> MATSRYEPVAEIGVGAYGTVYKARDPHSGHFVALKS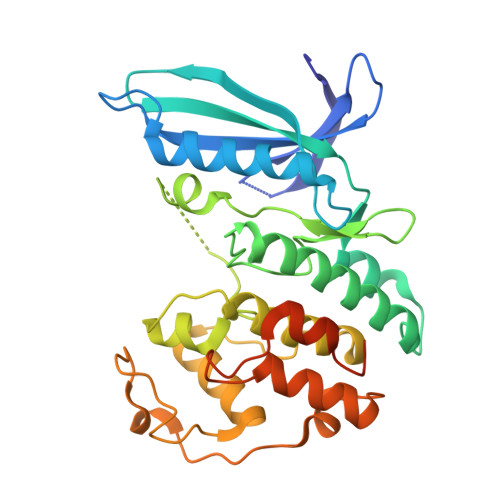VRVPNGEEGLPISTVREVALLRRLEAFEHPNVVRLMDVCATSRTDREIKVTLVFEHVDQDLRTYLDKAPPPGLPAETIKDLMRQFLRGLDFLHANCIVHRDLKPENILVTSGGTVKLADFGLARIYSYQMALTPVVVTLWYRAPEVLLQSTYATPVDMWSVGCIFAEMFRRKPLFCGNSEADQLGKIFDLIGLPPEDDWPRDVSLPRGAFPPRGPRPVQSVVPEMEESGAQLLLEMLTFNPHKRISAFRALQHSYLHKDEGNPELENLYFQGHHHHHH>[2x]TVRVRLAPSPTGNLHIGTARTAVFNWLYARHRGGKFILRIEDTDRERSRPEYTENILEGLQWLGLTWDEGPYFQSDRLDLYRQAIQTLLDKGLAYYCYCTPEELEALRAEQKAKGQAPRYDNRHRHLTPEEQAAFEAAGRTPVIRFKIEDDRQIEWQDLVRGRVSWQGADLGGDMVIARAAPRGEIGYPLYNLVVVVDDIAMGITDVIRGEDHIGNTPKQILLYEALGATPPNFAH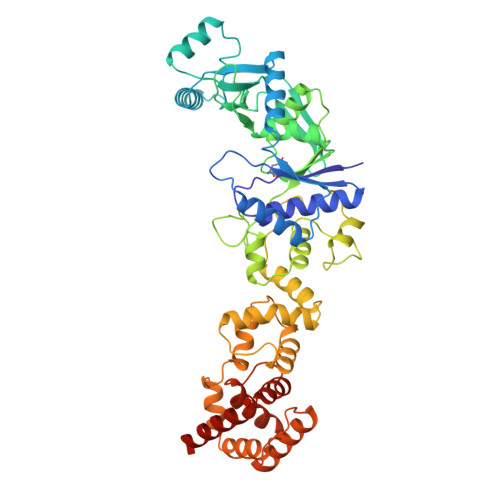TPLILNSTGQKLSKRDGVTSISDFRAMGYLAPALANYMTLLGWSPPEGVGELFTLDLAAKHFSFERINKAGARFDWDKLNWLNRQYIQQLEPEEFLAELIPLWQGAGYAFDEERDRPWLFDLAQLLQPGLNTLREAIDQGAVFFIPSVTFDSEAMAQLGQPQSATILAYLLEHLPAEPALTVAMGQQLIQQAAKAAGVKKGATMRTLRAALTGAVHGPDLMAAWQILHQRGWDEPRLAAALKQAQTTSLEHHHHHH> MAVNVYSTSVTSDNLSRHDMLAWINESLQLNLTKIEQLCSGAAYCQFMDMLFPGSIALKKV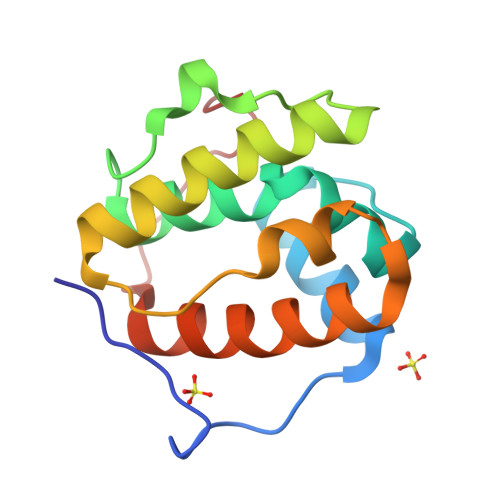KFQAKLEHEYIQNFKILQAGFKRMGVDKIIPVDKLVKGKFQDNFEFVQWFKKFFDANYDGKDYDPVAAR>MVKRMIALDGAQGEGGGQILRSALSLSMITGQPFTITSIRAGRAKPGLLRQHLTAVKAATEICGATVEGAELGSQRLLFRPGTVRGGDYRFAIGSAGSCTLVLQTVLPALWFADGPSRVEVSGGTDNPSAPPADFIRRVLEPLLAKIGIHQQTTLLRHGFYPAGGGVVATEVSPVASFNTLQLGERGNIVQMRGEVLLAGVPRHVAEREIATLAGSFSLHEQNIHNLPRDQGPGNTVSLEVESENITERFFVVGEKRVSAEVVAAQLVKEVKRYLASTAAVGEYLADQLVLPMALAGAGEFTVAHPSCHLLTNIAVVERFLPV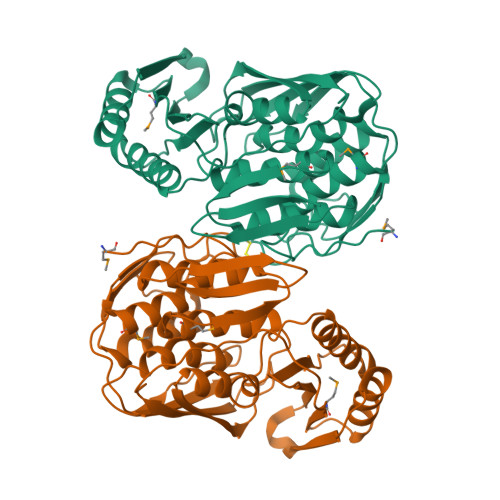RFSLIETDGVTRVSIEGSHHHHHH[4x]>[6x]MLNQELELSLNMAFARAREHRHEFMTVEHLLLALLSNPSAREALEACSVDLVALRQELEAFIEQTTPVLPASEEERDTQPTLSFQRVLQRAVFHVQSSGRNEVTGANVLVAIFSEQESQAAYLLRKHEVSRLDVVNFISHGTRKDEPTQSSDPGSQPNSEEQAGGEERTENFTTNLNQLARVGGIDPLIGREKELERAIQVLCRRRKNNPLLVGESGVGKTAIAEGLAWRIVQGDVPEVMADCTIYSLDIGSLLAGTKYRGDFEKRFKALLKQLEQDTNSILFIDEIHTIIGAGAASGGQVDAANLIKPLLSSGKIRVIGSTTYQEFSNIFEKDRALARRFQKIDITEPSIEETVQIINGLKPKYEAHHDVRYTAKAVRAAVELAVKYINDRHLPDKAIDVIDEAGARARLMPVSKRKKTVNVADIESVVARIARIPEKSVSQSDRDTLKNLGDRLKMLVFGQDKAIEALTEAIKMARAGLGHEHKPVGSFLFAGPTGVGKTEVTVQLSKALGIELLRFDMSEYMERHTVSRLIGAPPGYVGFDQGGLLTDAVIKHPHAVLLLDEIEKAHPDVFNILLQVMDNGTLTDNNGRKADFRNVVLVMTTNAGVRETERKSIGLIHQDNSTDAMEEIKKIFTPEFRNRLDNIIWFDHLSTDVIHQVVDKFIVELQVQLDQKGVSLEVSQEARNWLAEKGYDRAMGARPMARVIQDNLKKPLANELLFGSLVDGGQVTVALDKEKNELTYGFQSAQKHKAEAAH;>[7x]ALVPMVIEQTSRGERSFDIYSRLLKERVIFLTGQVEDHMANLIVAQMLFLEAENPEKDIYLYINSPGGVITAGMSIYDTMQFIKPDVSTICMGQAASMGAFLLTAGAKGKRFCLPNSRVMIHQPLGGYQGQATDIEIHAREILKVKGRMNELMALHTGQSL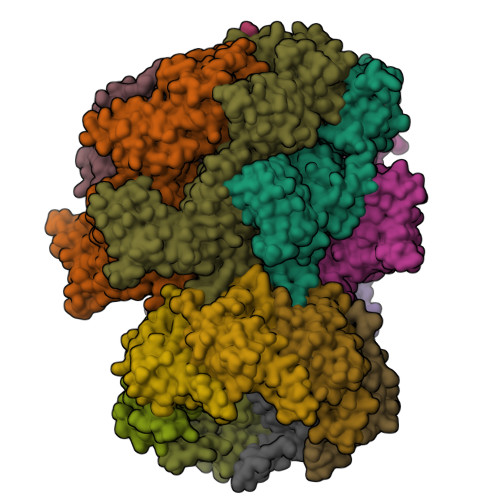EQIERDTERDRFLSAPEAVEYGLVDSILTHRNRSHHHHHH;> MGKTNDWLDFDQLAEEKVRDALKPPSMYKVILVNDDYTPMEFVIDVLQKFFSYDVERATQLMLAVHYQGKAICGVFTAEVAETKVAMVNKYARENEHPLLCTLEKA> TTIVALKYPGGVVMAGDRRSTQGNMISGRDVRKVYITDDYTATGIAGTAAVAVEFARLYAVELEHYEKLEGVPLTFAGKINRLAIMVRGNLAAAMQGLLALPLLAGYDIHASDPQSAGRIVSFDAAGGWNIEEEGYQAVGSGSLFAKSSMKKLY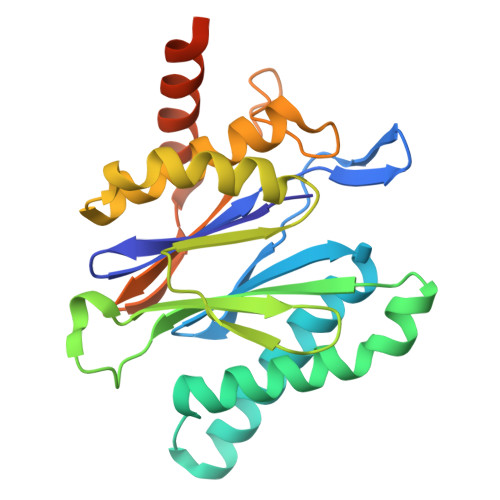SQVTDGDSGLRVAVEALYDAADDDSATGGPDLVRGIFPTAVIIDADGAVDVPESRIAELARAIIESRSGADTFGSDGGEKHHHHHH> GPNEQVSRSQQRGLRRVRDLCRVLQLPPTFEDTAVAYYQQAYRHSGIRAARLQKKEVLVGCCVLITCRQHNWPLTMGAICTLLYADLDVFSSTYMQIVKLLGLDVPSLCLAELVKTYCSSFKLFQASPSVPAKYVEDKEKMLSRTMQLVELANETWLVTGRHPLPVITAATFLAWQSLQPADRLSCSLARFCKLANVDLPYPASSRLQELLAVLLRMAEQLAWLRVLRLDKRSVVKHIGDLLQHRQSLVRSAFRDGTAEVETREKEP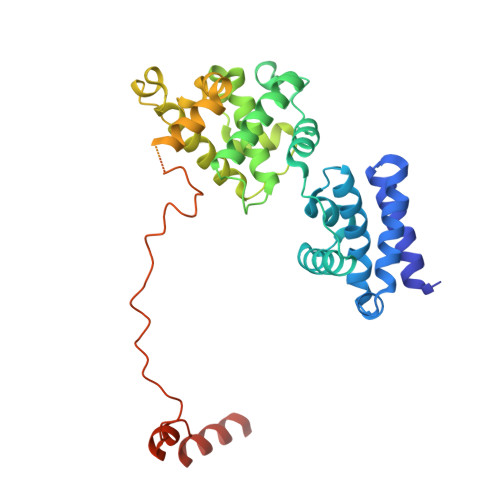PGWGQGQGEGEVGNNSLGLPQGKRPASPALLLPPCMLKSPKRICPVPPVSTVTGDENISDSEIEQYLRTPQEVRDFQRAQAARQAATSVPNPP>MRTGWATPRRPAGLLMLLFWFFDLAEPSGRAANDPFTIVHGNTGKCIKPVYGWIVADDCDETEDKLWKWVSQHRLFHLHSQKCLGLDITKSVNELRMFSCDSSAMLWWKCEHHSLYGAARYRLALKDGHGTAISNASDVWKKGGSEESLCDQPYHEIYTRDGNSYGRPCEFPFLIDGTWHHDCILDEDHSGPWCATTLNYEYDRKWGICLKPENGCEDNWEKNEQFGSCYQFNTQTALSWKEAYVSCQNQGADLLSINSAAELTYLKEKEGIAKIFWIGLNQLYSARGWEWSDHKPLNFLNWDPDRPSAPTIGGSSCARMDAESGLWQSFSCEAQLPYVCRKPLNNTVELTDVWTYSDTRCDAGWLPNNGFCYLLVNESNSWDKAHAKCKAFSSDLISIHSLADVEVVVTKLHNEDIKEEVWIGLKNINIPTLFQWSDGTEVTLTYWDENEPNVPYNKTPNCVSYLGELGQWKVQSCEEKLKYVCKRKGEKLNDASSDKMCPPDEGWKRHGETCYKIYEDEVPFGTNCNLTITSRFEQEYLNDLMKKYDKSLRKYFWTGLRDVDSCGEYNWATVGGRRRAVTFSNWNFLEPASPGGCVAMSTGKSVGKWEVKDCRSFKALSICKKMSGPLGPEEASPKPDDPCPEGWQSFPASLSCYKVFHAERIVRKRNWEEAERFCQALGAHLSSFSHVDEIKEFLHFLTDQFSGQHWLWIGLNKRSPDLQGSWQWSDRTPVSTIIMPNEFQQDYDIRDCAAVKVFHRPWRRGWHFYDDREFIYLRPFACDTKLEWVCQIPKGRTPKTPDWYNPDRAGIHGPPLIIEGSEYWFVADLHLNYEEAVLYCASNHSFLATITSFVGLKAIKNKIANISGDGQKWWIRISEWPIDDHFTYSRYPWHRFPVTFGEECLYMSAKTWLIDLGKPTDCSTKLPFICEKYNVSSLEKYSPDSAAKVQCSEQWIPFQNKCFLKIKPVSLTFSQASDTCHSYGGTLPSVLSQIEQDFITSLLPDMEATLWIGLRWTAYEKINKWTDNRELTYSNFHPLLVSGRLRIPENFFEEESRYHCALILNLQKSPFTGTWNFTSCSERHFVSLCQKYSEVKSRQTLQNASETVKYLNNLYKIIPKTLTWHSAKRECLKSNMQLVSITDPYQQAFLSVQALLHNSSLWIGLFSQDDELNFGWSDGKRLHFSRWAETNGQLEDCVVLDTDGFWKTVDCNDNQPGAICYYSGNETEKEVKPVDSVKCPSPVLNTPWIPFQNCCYNFIITKNRHMATTQDEVHTKCQKLNPKSHILSIRDEKENNFVLEQLLYFNYMASWVMLGITYRNKSLMWFDKTPLSYTHWRAGRPTIKNEKFLAGLSTDGFWDIQTFKVIEEAVYFHQHSILACKIEMVDYKEEYNTTLPQFMPYEDGIYSVIQKKVTWYEALNMCSQSGGHLASVHNQNGQLFLEDIVKRDGFPLWVGLSSHDGSESSFEWSDGSTFDYIPWKGQTSPGNCVLLDPKGTWKHEKCNSVKDGAICYKPTKSKKLSRLTYSSRCPAAKENGSRWIQYKGHCYKSDQALHSFSEAKKLCSKHDHSATIVSIKDEDENKFVSRLMRENNNITMRVWLGLSQHSVDQSWSWLDGSEVTFVKWENKSKSGVGRCSMLIASNETWKKVECEHGFGRVVCKVPLGPDYTAIAIIVATLSILVLMGGLIWFLFQRHRLHLAGFSSVRYAQGVNEDEIMLPSFHD[4x]

DEC-205 (CD205), a member of the macrophage mannose receptor protein family, is the prototypic endocytic receptor of dendritic cells, whose ligands include phosphorothioated cytosine–guanosine oligonucleotides, a motif often seen in bacterial or viral DNA. The MR protein family is characterized by a conserved domain architecture that comprises an N-terminal cysteine-rich (CysR) domain, a fibronectin type II (FNII) domain, and 8 or 10 contiguous C-type lectin-like domains (CTLDs). Here, DEC-205 is thought to function as a promiscuous endocytic receptor that captures a diverse repertoire of foreign and self-antigens and internalize them for antigen processing and cross-presentation. Namely, DEC-205, PLA2R, and the avian IgY receptor FcRY are all reported to exist in a compact conformation at low pH and transition to an extended state under basic conditions, although the mechanism of such rearrangements are unknown.

Building on this finding, we observed a large change in the elution profile of DEC-205 at pH 8.0, eluting with a mass four times that of the monomer, suggesting that in basic conditions DEC-205 formed a stable tetramer. We next performed cryo-EM analysis on the DEC-205 tetramer in basic conditions (pH 8.0). Here, the DEC-205 tetramer formed a 115 × 200 × 100 Å toroid shaped particle with a large central cavity and was ultimately resolved to 4.9 Å. The overall architecture of the DEC-205 tetramer revealed a major rearrangement of the second CTLD ring that enabled four protomers to assemble into a prolate toroid with clear D2 symmetry in the 2D class averages and final reconstruction. In contrast to the structural conservation of the first ring, the C-terminus underwent a dramatic rearrangement to form a tail–tail interaction along the median of the toroid. Within this extended confirmation, CTLD8 from one protomer contacted CTLD4 of the opposing protomer and vice versa. The cryo-EM reconstruction was unambiguous for the placement of the 10 (CysR to CTLD8) domains except for CTLD5. Here, the cryo-EM reconstruction suggests that CTLD5 is highly mobile within the tetramer, and the domain could act as an allosteric center for DEC-205’s pH-dependent rearrangements. As observed in the DEC-205 monomer, CTLD9 and 10 were absent from the final reconstruction, solidifying the notion that they are a highly dynamic part of the protein. Broadly the BSA of the protomer 1 and 2 head–head interaction accounted for ∼2300 Å2, whereas the protomer 1 and 3 tail—tail interaction was ∼1500 Å.> AFSWGSLWSGIKNFGSTVKNYGSKAWNSSTGQMLRDKLKEQNFQQKVVDGLASGISGVVDLANQAVQNKINSKLDPRPPVEEPPPAVETVSPEGRGEKRPRPDREETLVTQIDEPPSYEEALKQGLPTTRPIAPMATGVLGQHTPVTLDLPPPADTQQKPVLPGPTAVVVTRPSRASLRRAASGPRSLRPVASGNWQSTL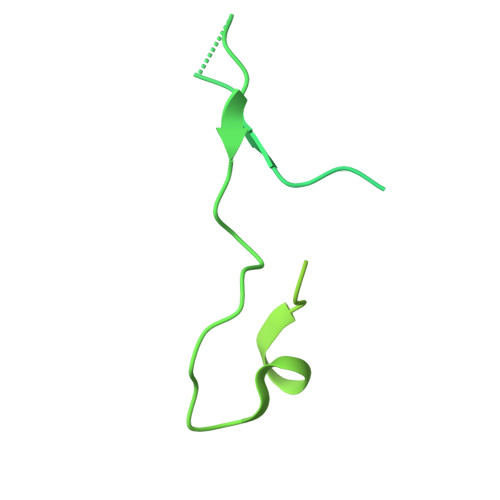NSIVGLGVQSLKRRRCF>GPKKKIQIMAEEALKDALSILNIVKTNSPPAEEQLERFAKRFERNLWGIARLFESGDQKDEAEKAKRMIEWMKRIKTTASEDEQEEMANAIITILQSWFFS[8x]

However, unlike IL-4, they signal strictly through the type I complex, offering insights into the intertwined functions of the type I and type II complexes.

We first grafted 14 cytokine residues implicated in the hIL-4–hIL-4Rα interface onto Neo-2, while preserving Neo-2 residues implicated in the Neo-2–hγc interface. The resulting grafted hNeo-4 was then subjected to random mutagenesis and four rounds of selection using the yeast surface display platform to increase hIL-4Rα binding. Clones from the converged library were expressed in Escherichia coli, and the molecule with the highest binding affinity for hIL-4Rα was selected (hereafter hNeo-4). Overall, 16 mutations were introduced into Neo-2 to derive hNeo-4; 1 of the 14 originally grafted mutations was modified by selection, and 2 more mutations were introduced during selection. The molecular structure of hNeo-4 was determined via X-ray crystallography to a resolution of 2.97 Å and showed atomic agreement with the computationally predicted model. The topology of hNeo-4 in complex with the hIL-4 type I complex was predicted using AlphaFold2, which showed the same overall topology as the native type I hIL-4 cytokine–receptor complex. Similar to previous reports, Kd values for hIL-4 binding to hIL-4Rα and the hIL-4Rα–hγc complex were 0.48 nM and 64 nM, respectively. hNeo-4 had a 121-fold weaker binding affinity toward hIL-4Rα (Kd = 58 nM) than hIL-4 due to a higher rate of dissociation (koff) and a slightly lower rate of association (kon). Interestingly, hNeo-4 had comparable affinity (Kd = 80 nM) for the hIL-4Rα–hγc complex to hIL-4. We validated that the Neo-2-derived hNeo-4 did not exhibit residual interactions with hIL-2Rβ or the hIL-2Rβ–hγc complex, confirming that the specificity was fully transformed. BLI binding studies confirmed that hNeo-4 did not interact with the type II complex.>[2x]SLWQFGKMINYVMGESGVLQYLSYGCYCGLGGQGQPTDATD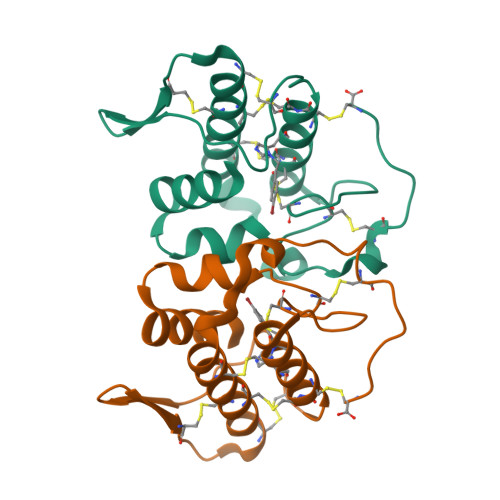RCCFVHDCCYGKVTGCDPKIDSYTYSKKNGDVVCGGDDPCKKQICECDRVATTCFRDNKDTYDIKYWFYGAKNCQEKSEPC> GEFELMEMIL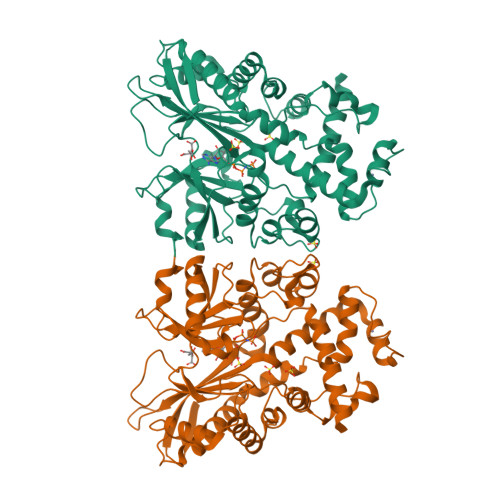EEKDASDWIYRGEGGANLVLAYAGSSPLFVGKVIRIQKARRNDKAIKNSNGVVSVLTSDEQHLWRENNELISSPNKEVLEQRYVQNVIIPLLGPKHVDAGVRVSVSKEFLECVDKKVTKQRPLARVNAANVDTSHDSALILNDHSLFSQGITSGGDCISVEIKPKCGFLPTSRFIGKENMLKTSVSRFKMHQLLKLEYIEISEESEYDPLDLFSGSKERVLEAIKALYSTPQNNFRVFLNGSLILGGSGESTGRTSPEIGYAFEDALKGFIQSEDGHRTECFLQLVSDAVYGSGVLDRLLEIQKLDKLDIEGAIHCYYDIINQPCPICREGRPLEAELSLHALPLDESLKIVKEYLIAATAKDCSIMISFQSRNAWDSEPSGDYVSLKPTNQTFDYKVHFIDLSLKPLKRMESYYKLDKKIISFYNRKQKAENTAEQIGNSKPSHS>SQSRIFYLRNFNNWMKSVLIGEFLEKVRQKKKRDITVLDLGCGKGGDLLKWKKGRINKLVCTDIADVSVKQCQQRYEDMKNRRDSEYIFSAEFITADSSKELLIDKFRDPQMCFDICSCQFVCHYSFESYEQADMMLRNAC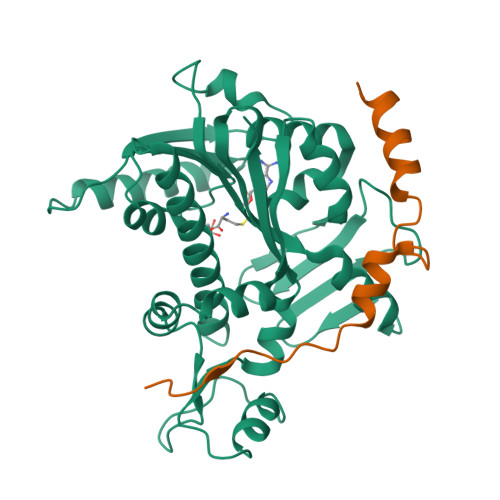ERLSPGGYFIGTTPNSFELIRRLEASETESFGNEIYTVKFQKKGDYPLFGCKYDFNLEGVVDVPEFLVYFPLLNEMAKKYNMKLVYKKTFLEFYEEKIKNNENKMLLKRMQALEPYPANESSKLVSEKVDDYEHAAKYMKNSQVRLPLGTLSKSEWEATSIYLVFAFEKQQ[2x];>TDTAEAVPKFEEMFASRFTENDKEYQEYLKRPPESPPIVEEWNS[2x]TERT-BUTYL 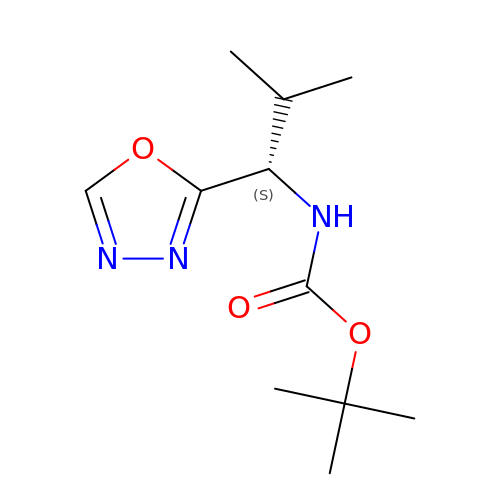[(1S)-2-METHYL-1-(1,3,4-OXADIAZOL-2-YL)PROPYL]CARBAMATE | C11 H19 N3 O3 | PARUDDGQWSBIIO-QMMMGPOBSA-N>LYIQNL[2x]

Aggregation-prone-motifs (APRs) of proteins are short segments, which – as isolated peptides - form diverse amyloid-like crystals. We introduce two APRs - designed variants of the incretin mimetic Exendin-4 - that both display crystal-phase polymorphism. Crystallographic and spectroscopic analysis revealed that a single amino-acid substitution can greatly reduce topological variability: while LYIQWL can form both parallel and anti-parallel β-sheets, LYIQNL selects only the former. We found that a simple change in crystallization temperature or modest changes of chemical composition of the solvent system (therefore the available interaction partners) can prompt formation of significantly different nanostructures: we identified four different polymorphs of the LYIQWL and two of the LYIQNL APR peptides.

In the present work we therefore synthesized the Trp5Asn mutant of LYIQWL and found that it forms a purely class 3 amyloid crystal structure. Crystals grown from both solvents contained β-strands of parallel orientation, but arranged in different amyloid topologies. In the monoclinic crystals grown from the ethanol containing solvent system, strands arranged in the class 3 topology could be observed, while the orthorhombic crystals grown in the absence of ethanol contained strands arranged according to the class 4 topology. While the class 4 structure did not contain any solvent molecules, the class 3 structure contained both water molecules and two ethanol molecules, one in a solvent channel near the chain termini and another wedged into the steric zipper interface. In the class 3 topology (monoclinic crystal) the same faces of the chains interact with each other, thereby forming two distinct zipper interfaces, namely that of Leu1, Ile3, Asn5 of chain #1 with Leu1, Ile3, Asn5 of chain #2, as well as Tyr2, Gln4, Leu6 of chain #1 with Tyr2, Gln4, Leu6 of chain #2. The assembly is stabilized by a hydrophobic cluster formed with Leu and Ile side chains complemented by “pure” Asn-Asn and Gln-Gln H-bond pairs. Finally, ethanol molecules insert themselves into the zipper interface through the formation of multiple H-bonds with both Gln and Tyr side chains. Tyr side chains also interact within the steric zipper interface in the class 3 crystal structure, here again with a displaced face-to-face geometry. Accordingly, we found strong and complex Asn5↔Asn5 and Gln4↔Gln4 interactions in the class 3 structure of LYIQNL, as they form H-bond networks “with themselves” in all three directions. However, it should be noted that in this crystal, the ‘odd interface’ (formed by Leu1, Ile3 and Asn5) is a dry one, that doesn’t contain a solvent molecule, and therefore this molecular architecture may be stable even without the ethanol molecule present.> APR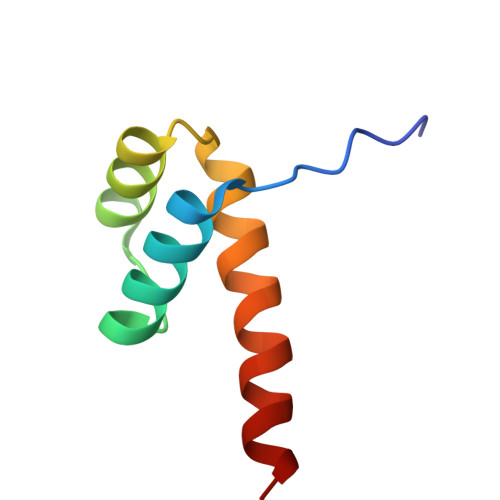KARTAFSDHQLNQLERSFERQKYLSVQDRMDLAAALNLTDTQVKTWYQNRRTKWKRQTAVG(2R)-2-(4-cyanophenoxy)propanamide | C10 H10 N2 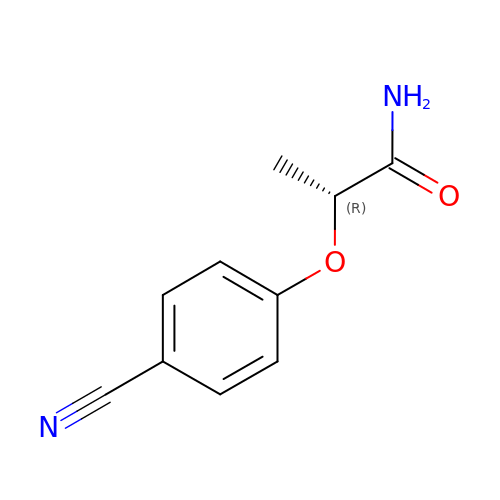O2 | JHIGQTTZYWLCKT-SSDOTTSWSA-N> MAYKRTFGHIPGHPEGSTYSNRRQVQKAGLHAHLQAGISGTAKQGADAIVLNGGYPDDRDYGDEIIYTGHGGQDPVTKKQIRDQDLDDPGNAGLVRSQLEGLPVRVIRGAGGEKPYSPSSGYRYDGLYKVVAHWFANHEDAPQFRVCQFQLVKIYDQVAAGVVVDNPDLSATAESTSVQGPAPHKKTTVSKAVRSAQVVKNVKGWHKHRCQVCGIVIEVDVGPYSQGAHIRPLGR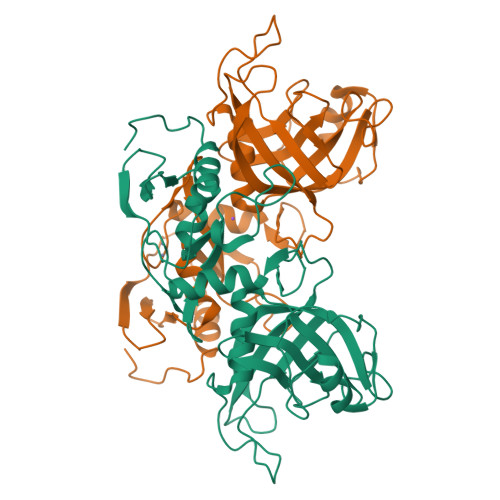KHGGPDVESNMLCLCPNDHVRFDNGALYITDDLKVVNALNGEVIGPLRVHPRHVIDLDHIRYHRSQLPNIPLEGSS>[6x]MKFALQINEGPYQHQASDSAYQFAKAALEKGHEIFRVFFYHDGVNNSTRLTTPPQDDRHIVNRWAELAEQYELDMVVCVAAAQRRGIVDEGEASRNGKDATNIHPKFRISGLGQLVEAAIQADRLVVFGD;>[6x]MSEVVKKFMYLNRKAPYGTIYAWEALEVVLIGAAFDQDVCVLFLDDGVYQLTRGQDTKGIGMKNFSPTYRTLGDYEVRRIYVDRDSLEARGLTQDDLVEIAFEDMETEEEFDN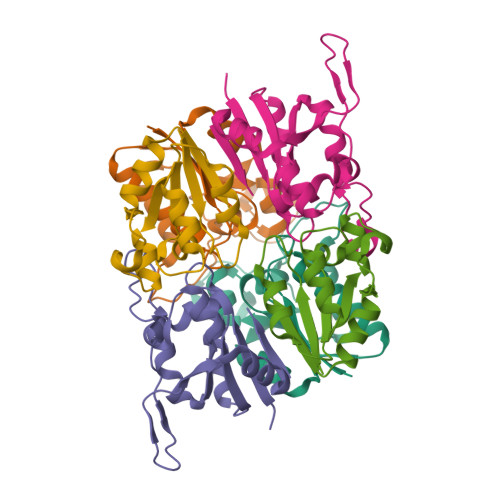IVEVIDSARVSELMNESDAVFSF;>MSILHTVNKSPFERNSLESCLKFATEGASVLLFEDGIYAALAGTRVESQVTEALGKLKLYVLGPDLKARGFSDERVIPGISVVDYAGFVDLTTECDTVQAWL[6x]> MLRITLLVVGRAPPVIGCTRKARYAGIDDNPTITYKPWDTTEPLMADYGWTRGKLPKFRARSPFHRQQIARRMVTEMIRKDYCIVGGARAPALRILADHVVELAKAGDTDS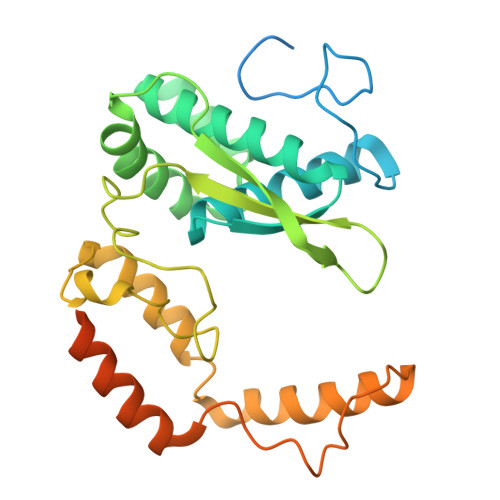RQQLAYFLHDPLMVDKAFDEYPRRFKDMNAKYAMMTRLKSRRRTDAVAMYFVEYKNRDMSDNHKGEDYSAGPERFFLPPRIVETEKGIQRPPHMQMAFDRWASKFKTEEFHHWWRLRHAKLRYWGVRNVPHPSDVDPLWTEKEEEEWHNEMLANTGEYEDLDLDDESYTAAGEGGEPSPAGDGPQPQRVG>MSVLFISDLNLEAERPDITRAFLSFLDERARRAEALYILGDFFEAWIGDDGMDAFQRSIAQSLRQVADGGTRIYLMHGNRDFLIGKAFCREAGCTLLPDPSVIDLYGEPVLLMHGDSLCTRDEAYMRLRRWLRNPLTLWVLRHLPLATRHKLARKLRKESRAQTRMKAVDIIDVTPEEVPRVMRGHGVRTLIHGHTHRPAEHPLDIDGQP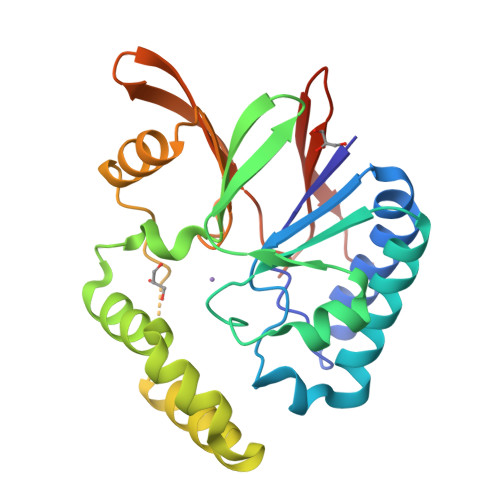ARRIVLGDWDRQGWALEIDANGHRQAPFPLLEHHHHHH[2x]> MSDIFNSPQNKASILTALMKSTTGDVEDVLIPKRFRPAKDPLDSPQAAAQFLKDNKYRILRPRAIPTMVELETDAALPRLRQMVEDGKLKDTVSVPEGTTAFYPKYYPFHKPDHDEVGTFGAPDITLLKQLTFFLLENDFPTGPETLRQVREAIATLQYGSGSYSGQLNRLLAMKGVATGRNPNKTPKTVGYTNEQLAKLLEQTLPINTPKHEDPDLRWAPSWLINYTGDLSTDKSYLPHVTIKSSAGLPYIGKTKGDTTAEALVLADSFIRDLGRAATSADPEAGVKKTITDFWYLSCGLLFPKGERYTQVDWDKKTRNIWSAPYPTHLLLSMVSTPVMNESKLNITNTQTPSLYGFSPFHGGMDRIMTIIRDSLDNDEDLVMIYADNIYILQDNTWYSIDLEKGEANCTPQHMQAMMYYLLTRGWTNEDGSPRYNPTWATFAMNVAPSMVVDSSCLLMNLQLKTYGQGSGNAFTFLNNHLMSTIVVAEWVKAGKPNPMTKEFMDLEEKTGINFKIERELKNLRETIVEAVETAPQDGYLADGSDLPPIRPGKAVELDLLGWSAIYSRQMEMFVPVLENERLIASAAYPKGLENKALARKPGAEIAYQIVRYEAIRLVGGWNNPLLETAAKHMSLDKRKRLEVKGIDVTGFLDDWNNMSEFGGDLEGITLSEPLTNQTLVDINTPLDSFDPKARPQTPRSPKKTLDEVTTAITSGTYKDPKSAVWRLLDQRTKLRVSTLRDQALALKPASSSVDNWAEATEELA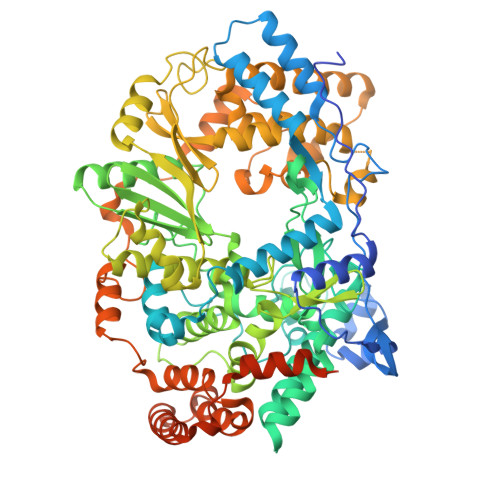QQQQLLMKANNLLKSSLTETREALETIQSDKIIAGKSNPEKNPGTAANPVVGYGEFSEKIPLTPTQKKNAKRREKQRRNQVEHHHHHH1-beta-D-glucopyranosylpyrimidine-2,4(1H,3H)-dione | C10 H14 N2 O7 | 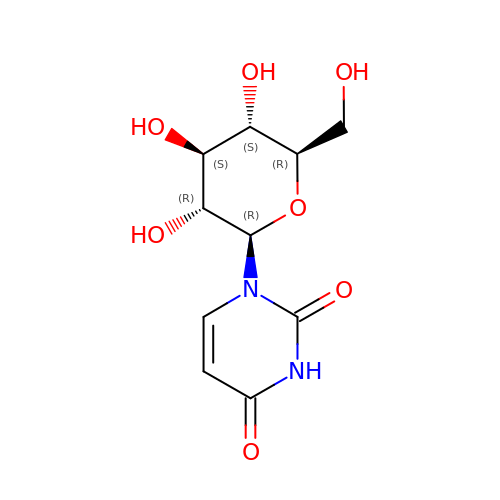PBGBADORVLQASN-DDIGBBAMSA-N>GASTAQPKQEAYIQSTELFLQNKYSDVITTLEDYAPEDMPYVIQYELASSYVMTESLTEEQRQTVSNNITLKTDEQYMLYWIYIGRSQSEEALELARTIEDRDLIVYALLKYREQIKGDTDLSGDEKQKKLDEIDQEIKEYERERKESEAQLEEEQQSEQQ[4x]

The membrane-bound EssB is an integral and essential component of the bacterial type VII secretion system that can contribute to pathogenicity. One of these is EssB, a 50-kDa bitopic integral membrane protein that is conserved among T7SS gene clusters in Firmicutes. The architecture of Geobacillus thermodenitrificans EssB has been investigated by combining crystallographic and EPR spectroscopic methods. The protein forms a dimer that straddles the cytoplasmic membrane.

A higher resolution structure of EssB-CΔ, residues Ala241 to Gln397, resulted when the flexible C terminus was omitted from the recombinant polypeptide. Approximately 75% of residues are in α helices arranged into a series of coiled-coil motifs that are predicted to extend across the cytoplasmic membrane. The structure starts at α1, with Ala241 at the transmembrane border, potentially the continuation of the helix that transcends the membrane. At the lower end of α4, a sodium:malonate ion pair is bound. The asymmetric unit of EssB-CΔ consists of four molecules, which are labeled A to D. An average rmsd value of 1.38 Å is obtained from the least-squares fit of the Cα positions of individual subunits with each other. The dimer is primarily formed by interacting residues on α1, α2, and the loop linking α4 to α5. However, with a solvation free energy gain of −14 kcal/M (estimated using PISA; Krissinel and Henrick, 2007), the dimer is predicted to be thermodynamically stable. The extracytosolic E273C showed a major distance distribution of 44 Å, compared to the value of 43 Å derived from the EssB-CΔ crystal structure, essentially confirming the assigned dimer structure and ruling out the physiologic relevance of the crystallographic dimer contained in the asymmetric unit (AD pairing) with a theoretical interspin distance of 49 Å. The topside surface exhibits two large grooves, one formed between α4 and α8 and one between the helix pair α3-α4, above the dimer interface.> MSKMSDVKCTSVVLLSVLQQLRVESSSKLWAQCVQLHNDILLAKDTTEAFEKMVSLLSVLLSM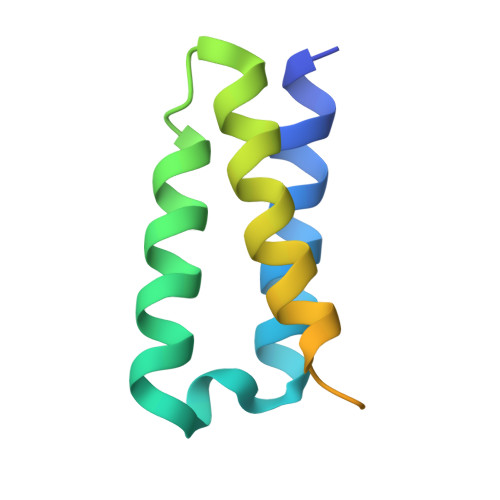QGAVDINKLCEEMLDNRATLQHHHHHHHH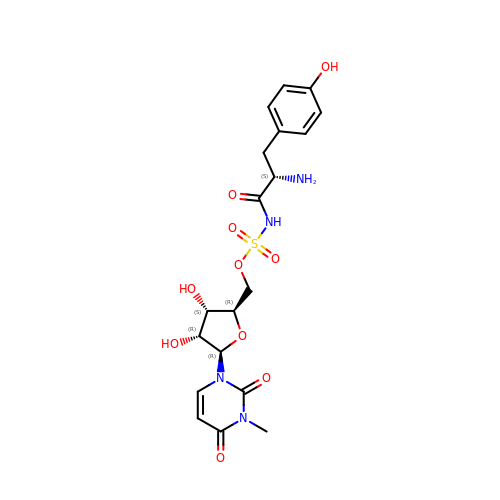[(2~{R},3~{S},4~{R},5~{R})-5-[3-methyl-2,4-bis(oxidanylidene)pyrimidin-1-yl]-3,4-bis(oxidanyl)oxolan-2-yl]methyl ~{N}-[(2~{S})-2-azanyl-3-(4-hydroxyphenyl)propanoyl]sulfamate | C19 H24 N4 O10 S | JZICRHJSYJTEMP-IQNGCQKYSA-N>MSLRPCFVSLIDESDKPILIYVPNEAENEMNDVLKYNVLSNISLDYFESALVEWHSLDSKPLLKSIFQLEGVSVFAMLIKQTGLKIVIGFEQKSLSGADDEFEAINQIFETVRKIYIRVKCNPLLVSGDE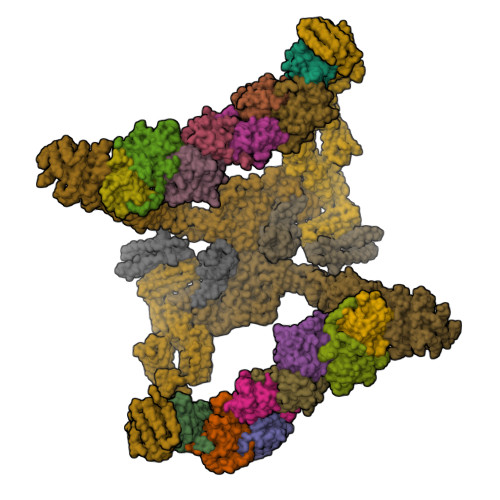KSIIKSLERKFDELFISTEVEL[2x];>[2x]MSSTHSNNVGHPQSSPQGPLTEQQRAQQQYQIFENSLPKVSQSVYQMLLNEMVPLAMGIERQISGDVISSDSNVTSENGNINNMIKRLKIEEHHTVDIIRSHNLIHELYKADEEEKEKVLARLRNIGFQIGLKLSELLIFSNNPNLKFKEMDLLLIMKFICRDVWKQIFGKQIDNLKTNHRGTFYLLDYDYRPIQSFSLEEDAKNEELKMIEPFLEIPVGIIRGVLSSLGYSSEEVICLASFIDRPTDRPKTAFPKGVSFHVQVTMPQ;>MVSTTQSRSLKAMGEEIWKNKTEKINTELFTLTYGSIVAQLCQDYERDFNKVNDHLYSMGYNIGCRLIEDFLARTALPRCENLVKTSEVLSKCAFKIFLNITPNITNWSHNKDTFSLILDENPLADFVELPMDAMKSLWYSNILCGVLKGSLEMVQLDCDVWFVSDILRGDSQTEIKVKLNRILKDEIPIGED[4x];>MGIYSFWIFDRHCNCIFDREWTLASNSASGTINSKQNEEDAKLLYGMIFSLRSITQKLSKGSVKNDIRSISTGKYRVHTYCTASGLWFVLLSDFKQQSYTQVLQYIYSHIYVKYVSNNLLSPYDFAENENEMRGQGTRKITNRNFISVLESFLAPMVNQ[2x];>MAIETILVINKSGGLIYQRNFTNDEQKLNSNEYLILASTLHGVFAIASQLTPKALQLTQQTNIENTIPYIPYVGMSSNRSDTRNGGGNNNKHTNNEKLGSFKGDDFFKEPFTNWNKSGLRQLCTDQFTMFIYQTLTGLKFVAISSSVMPQRQPTIATTDKPDRPKSTSNLAIQIADNFLRKVYCLYSDYVMKDPSYSMEMPIRSNLFDEKVKKMVENLQ[2x];>MSQRIIQPSASDQQFPGKSDGYEYTVGPKQAITSEASTTYIPSRIYSESLLFKRQEASLSAMAFLFQEMISQLHRTCKTAGDFETKLSDYGHNIGIRLLELLNFRASSSPSSLPRASAFLSQNESSSKLSNASNSPGMLANSSTATSASANERLQEKQTESLSNYITKMRRRDLKILDILQFIHGTLWSYLFNHVSDDLVKSSERDNEYMIVDNFPTLTQFIPGENVSCEYFVCGIIKGFLFNAGFPCGVTAHRMPQGGHSQRTVYLIQFDRQVLDREGLRFG[2x];>MPQYFAIIGKKDNPVYEIEFTNAENPQGFPQDLKELNPFILHASLDIVEDLQWQINPTSQLNGNGGNGSNGGGGFLRSRAVNNTDNCYLGKVDHFYGLAITAYISYSGMKFVMIHGNSANSSVVIDDNNMRSFYQEVHELYVKTLMNPFYKITDPIRSPAFDSRVRTLARKHLSK[2x];>MDKEIYCGSVPVSYFDPFDLFESLRPEFQQILPLDNIHWKAFDGTVRTVNRLPIELIPEGRGEADKSNDEQPFIRFLIVNCISIDQYRAKVRPLVRQWLPNLESVSSSTGEKMIYKPIILLYANSEVVDSNLFKSVSLMEKFGKDFPHVQTLEVRSVYRSPKERQEFWNQFSQKIKASVLSIFQKRLTHLQHSLANLQKGNNFEEQLLTREKLYELYVVFNILEDASLELQKIKKEILRRNMNMPDGKLQVPFESSSKSDESLGSIIIEGTLDKFQLHKYFFIRRLRLLKLEDQTLTAFVGAFQLIKNFIESISIEYRKSVRLLEFKHYFITSMLSYFEFENVSNPLLCEIKAELLMLKRDNWVQGVMATSGYRLMDKNYPNSDVKYKFDLLKETFVDETVFQENFLTLTKEILSLFNKCEGKRQRIVDILSIEIGLLYYQGKKYEEAVSLFLSCYEYYTQTNWNSIGLKILQVFIDSLSHCPKLDVLQIDGESVSASAVLTNAFLNILKLCKDNDSKEIWWKKFMDLQMKNNIHLMYPLDGLFEVTLNSKVHLARANVSAIEVNLKSYGFPEDISTKTMRLSLKNMGGDVIVFGASDFLLKKGENKLILECRDIMYGEFSLLSFEIIVEGITFVKEFPENQDEFIVVPEIYCKESTKVLVKQAHNLNLGEYALELKSVQSDALESLQVEVEVQKNIGNMKNLPVSFSMDEIQARKRYNTPFENVRLEYYLLDQITAFDLIIKTSFTKKNDQGTFGETKKVRIQCYLQLSVSVEDIFKKDIFFFKFLLNSSVREEPVILYSSELSAPDTRNDYNIRGDYIATTPALITFDGNESFINCYEITANNNFDSKDIFNLKVRYNTLKEQLDCFITDAVLIEGDVEWFILFEKWKTFWELEILKKLKYDYDAFKENRIIRLLKTSIDLNKTKSKIRNLCIEKAVLDKILICLNKVSRGIAVCNTDMDEYVRNLVPKQLTVPVQLPGFEQFFHVQFEQMETSHDALHDTIATIGNSLSYTVIVENLSGQWGQDVIDDGGYIFEILSSNEWLIHGQKRCAIKEKRKEFEVHLIPLKKGYLNFPRVEITNINGKSCRVDHSNAFESILIF[2x];>[2x]MNILKHFPSYVGPSKIRTLVIPIGHWTRKEFNNAVQKLSEFNEIHLSDVTPIDSPIFTPQGFPHGKLFFDFLTIDHDDALELFLYDFEPFRKTFVIIGLVNDYSDPLTNLNFMKEKYPTLISPNLVYASSTPTKELEQTIDTMENVFASSPDMQKNIETIMCDIARNFLTALNSYYSSYKHVTLRSPGAIGGNAVLKTTLIRQNSYTSSSSSTPMSAVQSSVSSSSKAGSVTTASKRLSSFEMTTNSLKRSASLKLATTLSTSENRSQQKSLGRQMKILGNFQLLAGRYVDALNSFVDAITTLYKVRDYLWLGSALDGISICFLLLSYLGLSYQIPQIVSLICPVEKLNFESSSTGISPVDSNSKATASTTASSTPRNSISIAAMQSPRNSIMSLSAPALNIDVENINLPLLIKCISDKVLYYYDLSLMHNSEYAPQVVYCEFLLKTLTFMTSCYKSSEFSKDVLDNIVKNQHRALSDIPNSPMFPRFEVYFYSNKLFELQLKEMQVEAQIKIYSTMAEVYRLLGYKRKQLFVLRLLMVALLATPNKIAWHPDYRTLIDTIIELLNINESEAKINVDDPSQSTWLILQKKILQLCIKVSRKINDFEYVAKFSSILITKYTHLLNQSEQDALFKEYIQPSITNESITSYWDPFILREVVINRILDSDPTSNEIPLESDVSSLESLENRQKTQDINPQEVFNPFKRVQPTSFVSNNSTKVPILVFLVGDKAEFTCRVQNPFKFDFTINDIQLDEEISEFCEIDRKAVSYSGPYNVKAESIRSITLPLIIKKPTYKKIYEISCLKISILKLPLQKFDIINDSRRSNPVEEEAEYSKCIYGKLKIKILPEQPQLELLSTSKMTRNSWMMLDGTKTDFHITVRNKSLSCAINHIKIIPMNNIEQMLKPDYWKKMPPDDLYIMEKQLDWLSKSCVRIIKLPTVIKPNETITFDLELDNTAVPFNFTGFDLLIEYGMSATDESCIYLKKLSIPYEVTLRRTIEVPSMDIIPLNELFSSQVENVDWIEYVMSKIRAESNLHSRDFILLLLDFRNSWIDGIKLNVQFEDFTSNEYHVEASHTSRIIVPIKKIDYKKYNFENTPIPRIFPGRQFIQSGLNEEQTIEMRQKFWCREHIISKLKCNWKLTTDQSVTGSVDFNKFIEKFDHKMVYTIYPGRLFYGVQLLLDEPKVKVGEIINLKIITEPTSTCRRKQNSTVNFLDIVIFDSKTSKILPRSNRRILYNGSLTKPISTTKVSEINLEIIPIEKGRYEFSVCISKSNNQDGIIQFDSENVILSVI;>[2x]MECFVPLRCDLDGSNIEQLRQSHLSRKFIIFDEQLNLWLWFQGNSQENKRFVLQNMIILINEAQVTRTSTIDDYFTQVENNENLWRLKNDCCSKILFKSNVVMNNGYNNQIKFVFEYKSVDANFNNQDSLQDPQAKYTLDKYSSEEILPSFEPVYSWSSAATKSSKNTNNHLEKNNRATHRVSSKNSEVHEADVSRNPNTFTLKLQYPIFSLLNMRLRNISLKSEHCILSSLDFQTSKASEQLTKKFIYPQEHNSFLKLNFQEISYKLIDGTSQIELDPICPLKVPLTAFSYDSISATFKLVLLPKSTQPHRVKITLAYELELHPNLKLPVRTSWETEVTLKRSMPISSTSSQYSSNNNNTNHSASFNGAANNVNSGGLANLRLGGVSSSRFSLGAASTTSLVNSKLSNVKFKFINSNIKVIKGEKFTMRLQIINSSSSPLDLVVYYNNTINPIPSANNVRNSNGINNCGMNNGTIPNSPLTLENQYQLHNKYRKIAEGIILLSNDYKIPVVPPRETYFADLRFIGIMSGYYGTLSGLKVLDLNTNELIEVGNGASVLIQ>[2x]MNQKAVILDEQAIRRALTRIAHEMIERNKGMNNCILVGIKTRGIYLAKRLAERIEQIEGNPVTVGEIDITLYRDDLSKKTSN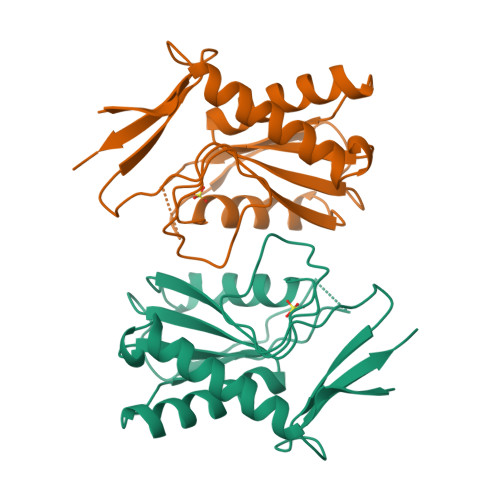DEPLVKGADIPVDITDQKVILVDDVLYTGRTVRAGMDALVDVGRPSSIQLAVLVDRGHRELPIRADYIGKNIPTSKSEKVMVQLDEVDQNDLVAIYENE methyl alpha-L-fucopyranoside | C7 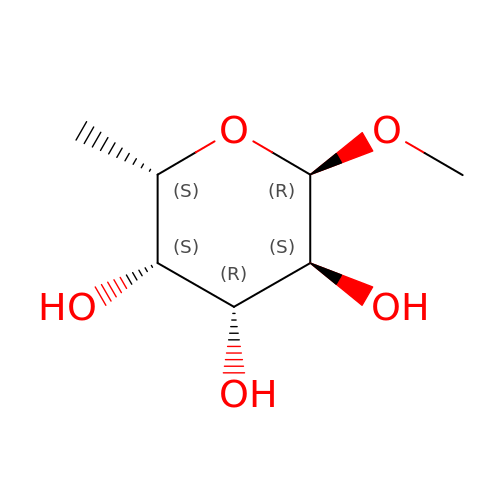H14 O5 | OHWCAVRRXKJCRB-CXNFULCWSA-N>[7x]GSMAKVQVNNVVVLDNPSPFYNPFQFEITFECIEDLSE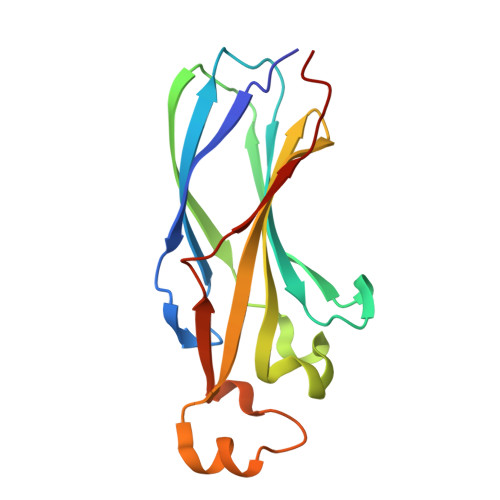DLEWKIIYVGSAESEEYDQVLDSVLVGPVPAGRHMFVFQADAPNPGLIPDADAVGVTVVLITCTYRGQEFIRVGYYVNNEYTETELRENPPVKPDFSKLQRNILASNPRVTRFHINWED PICEATANNOL | C14 H12 O4 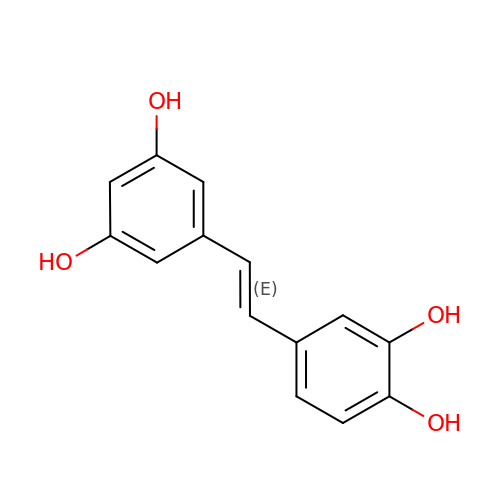| CDRPUGZCRXZLFL-OWOJBTEDSA-N>MKITVLVGGVGGARFLLGVQNLLGLGSFADGPSKHELTAVVNIGDDAWMHGVRICPDLDTCMYTLGGGIDPDRGWGHRNETWNAKEELAAYGVQPDWFGLGDRDLATHLVRSQMLRAGYPLSQVTEALCKRWQPGARLLPASDERSETHVVITDPTDGERRAIHFQEWWVRYRAKVPTHSFAYVGADQATAGPGVVEAIGDADIVL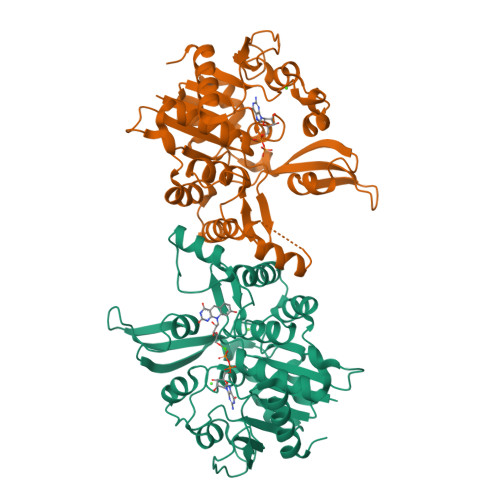LAPSNPVVSIGPILQIPGIRGALRSTSAPVIGYSPIIAGKPLRGMADECLKVIGVESTSQAVGEFFGARAGTGLLDGWLVHEGDHAQIEGVKVKAVPLLMTDPEATAAMVRAGLDLAGVSL[2x]> NLYPD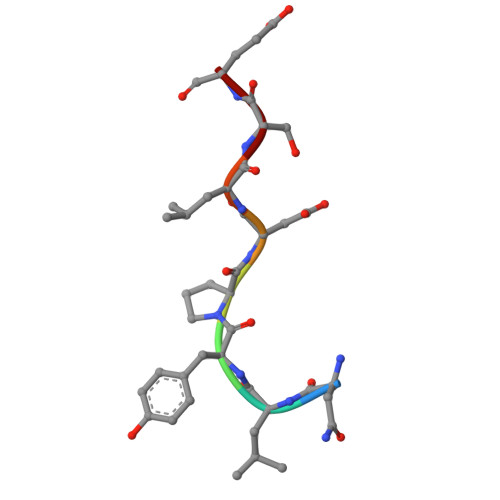LSE>[2x]MAFELSPSDLEPLLQGACFFGSGGGGTMISARHLAANFRKGDYYPTDKVRVVDVDEATDGDCVMVAYMGAPDAINQVQWPNGPVEAALAA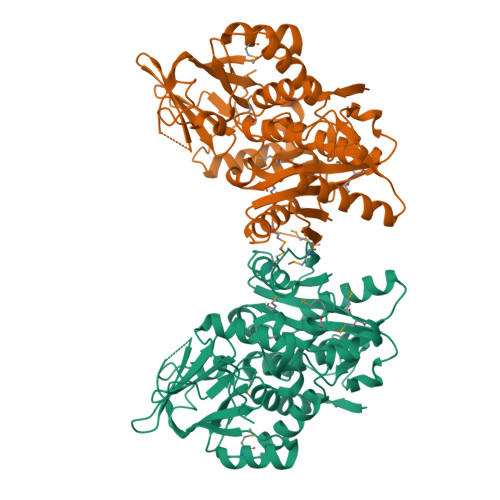RQRLESQGRKLAYVVAPESGALGFVVASLVAAKLGLAVVDADGAGRAVPSLPMLTYAAAGVPPTPAFLAGESGLCVELGVRMPPPDGQRREDISTVVEQMLRPILTNPQFGQFGGLAMWMMSPAQLGGALPVRGTLSRALKLGRALQDGKVKTAEAMLDFLRRELDIKGKLLFGPATLASPEVSTAGGFDLGKVVLEDGERRCTVLYQNESLLAWDSALSHPLATAPDAISYFVEGEGQHVFSNGDLSGNDHGLDPSVRGRKAAVIALPAAAPLSEGLILQSFADELAQLGYLGPYAPVDAGRERARLEHHHHHH>MKLKKIVFTLIALGLFSCKTTSVLVKNEPQLKTPKNVILLISDGAGLSQISSTFYFKSGTPNYTQFKNIGLIKTSSSREDVTDSASGATAFSCGIKTYNAAIGVADDSTAVKSIVEIAALNNIKTGVVATSSITDATPASFYAHALNRGLEEEIAMDMTESDLDFFAGGGLNYFTKRKDKKDVLAILKGNQFTINTTALTDFSSIASNRKMGFLLADEAMPTMEKGRGNFLSAATDLAIQFLSKDNSAFFIMSEGSQIDWGGHANNASYLISEINDFDDAIGTALAFAKKDGNTLVIVTSDHETGGFTLAAKKNKREDGSEYSDYTEIGPTFSTGGHSATLIPVFAYGPGSEEFIGIYENNEIF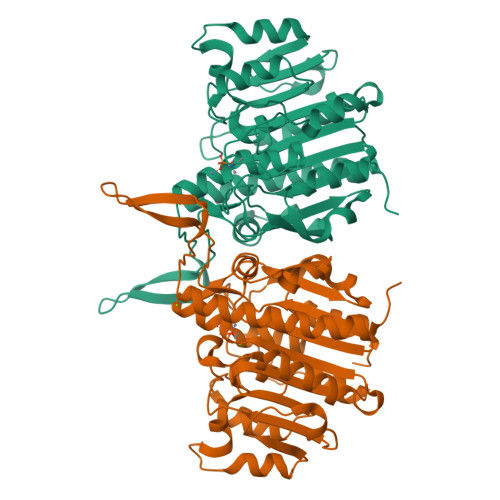HKILKVTKWNQ[2x]2,4-dimethyl-5-[[2-(4-methylpiperazin-1-yl)phenyl]methylamino]pyridazin-3-one 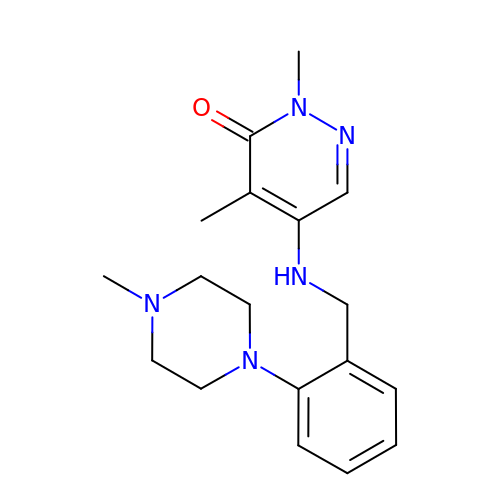| C18 H25 N5 O | HONYBLSJNSYWKQ-UHFFFAOYSA-N> MKAELRAKEYFDDRATREMAEHLKGAKRSYKETLAYACRILAMTGQEAGLAGQISFRSERPNAYWTLRFGLGFDEATPDDFIEVDRDLNTLTGEGMANPATRFHLWVYDARPDVKSLIHTHSPWASALAAARQPLVIAQMDMTPLHDDCAFLGEWPGVPIADQEGVLISEALGRKRAIILAHHGYLTAGVSIEEATYLSVYLERAARMQIRAQAFGPLTPVDDALAKEAHDYLLKPSIVGATFDYWCRQTHSAGPAAKHHHHHH

The enzyme responsible for the core function of heterotrophic nitrification is pyruvic oxime dioxygenase (POD). POD is a non-heme, Fe(II)-dependent enzyme that catalyzes the dioxygenation of pyruvic oxime to produce pyruvate and nitrite. Bacteria of the genera Alcaligenes and Pseudomonas are known to perform heterotrophic nitrification, which produces nitrite from ammonia using pyruvate oxime (PO) as an intermediate metabolite. PODs have additional sequences at the N-terminus consisting of 20–30 amino acid residues that are not present in class II aldolases, corresponding to the disordered region of AfPOD in its crystal structure.

The structure of AfPOD and its homologous enzyme BWPOD were very similar to those of class II aldolases, whereas the zinc ion, which is the active center in other class II aldolases, was replaced by Fe(II) ion in the active state of AfPOD. Interestingly, a homology search using the KEGG genome database revealed that many class II aldolase genes with unknown functions shared extremely high sequence homology (E-value < e-60) with AfPOD. Molecular phylogenetic analysis has shown that these proteins form a monophyletic group that is distinct from other class II aldolases such as FucA, and recombinant experiments have confirmed their POD activity. Initially, we expected the flexibility of the region to cause disorder in the N-terminal sequence of AfPOD and BWPOD crystals, but the AlphaFold2 prediction gave an α-helix conformation in the sequence.>[2x]RGSHMEKLAKNKVISIDAGRKYFTLNQLKRIVDKASELGYSDVHLLLGNDGLRFLLDDMTITANGKTYASDDVKKAIIEGTKAYYDDPNGTALTQAEVTELIEYAKSKDIGLIPAINSPGHMDAMLVAMEKLGIKNPQAHFDKVSKTTMDLKNEEAMNFVKALIGKYMDFFAGKTKIFNFGTDEYANDATSAQGWYYLKWYQLYGKFAEYANTLAAMAK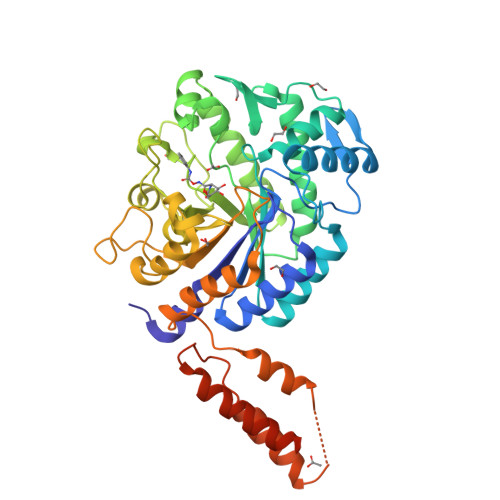ERGLQPMAFNDGFYYEDKDDVQFDKDVLISYWSKGWWGYNLASPQYLASKGYKFLNTNGDWYYILGQKPEDGGGFLKKAIENTGKTPFNQLASTKYPEVDLPTVGSMLSIWADRPSAEYKEEEIFELMTAFADHNKDYFRANYNALREELAKIPTNLEGYSKESLEALDAAKTALNYNLNRNKQAELDTLVANLKAALQGLKPAVTHSGSLDENEVAANVETRP The Tad (Tight adherence) pilus is a bacterial appendage implicated in virulence, cell-cell aggregation, and biofilm formation. Our analyses reveal that RcpC forms a dodecameric periplasmic complex, anchored to the inner membrane by a transmembrane helix, and interacting with the outer membrane secretin RcpA. Collectively, these data demonstrate that RcpC forms the Tad pilus alignment complex, which provides a conduit across the periplasm for the Tad pilus filament to access the extracellular milieu. A structural model of RcpC, combined with transmembrane domain analysis of its primary sequence, predicted that RcpC is comprised of an N-terminal TM helix, followed by two folded domains (D1 and D2) and a C-terminal β-hairpin that localize in the periplasm.

Further processing of the dataset, including imposing 6-fold symmetry, yielded a 2.5 Å resolution Coulomb potential map of the RcpCΔN dodecamer. Using this map, we were able to build an atomic model of RcpC33-303 containing twelve copies of RcpC. From this model, we determined that the RcpC dodecamer has a diameter of ~15 nm, and possesses a ~5 nm pore at its centre. Remarkably, the Tad pilus filament has previously been reported to have a diameter of ~4.5 nm, indicating that it is could transit through the RcpC pore. Interestingly, the D1 domains are arranged into six dimers, whereby each domain only interacts with one other D1 domain, whereas the D2 domains are structured as a dodecameric ring with C12 symmetry. Accordingly, RcpC adopts two distinct conformations in this structure, which differ in the relative position between D1 and D2, explaining why the overall symmetry of the complex is C6. Although present within the sample, there is no density for the C-terminal β-hairpin domain, which we could not resolve in spite of extensive 3D classification and masking strategies. The overall structure of RcpC demonstrates that individual subunits are twisted around the central pore with the D1 domain of each subunit primarily forming contacts with the D2 domain of the neighboring RcpC subunit. Additionally, L3 forms molecular contacts with the D2 domain of the adjacent RcpC molecule. These interactions lead to a very extensive interface between RcpC subunits, measuring ~2400 Å2 within dimers and ~1930 Å2 between dimers, which collectively are comprised of four distinct interfaces.

>MNAHAPSVAPASATVDASLEKLERKPVLVASRDLPALAVIGRDDLSVELLRTAPVGSYDRPEALLGKRVWVAVPAGSILSAATLEPGGPLARTIRPDERAMAIAVDEVVGGGGFVLPGDYVDVMLFVRDERDGESTPLAQLVLPGVRVLTYGERIAVGSDGQDRSNQEKDPRPPRTAVLAVPEDGVARLMLASQAGSLRLAIRSKDEELYRREQEGALLQASLGAPSAALSLDQLLERRKPTAPSVRSAAPRVPVANGVTVYRGSAMTHEAPLEHHHHHH[12x]>MGNYDSTPIAKSDRIKRLVDHLYAKMPEIEAARAELITESFKATEGQPVVMRKARAFEHILKNLPIIIRPEELIVGSTTIAPRGCQTYPEFSYEWLEAEFETVETRSADPFYISEETKKRLLAADAYWKGKTTSELATSYMAPETLRAMKHNFFTPGNYFYNGVGHVTVQYETVLAIGLNGVKEKVRKEMENCHFGDADYSTKMCFLESILISCDAVITYANRYAKMAEEMAEKETDAARRQELLTIARVCKNVPEFPAESFQEACQSFWFIQQVLQIESSGHSISPGRFDQYMYPYYEKDLKEGSLTREYAQELIDCIWVKLNDLNKCRDAASAEGFAGYSLFQNLIVGGQTVQGRDATNDLSFMCITASEHVFLPMPSLSIRVWHGSSKALLMRAAELTRTGIGLPAYYNDEVIIPALVHRGATMDEARNYNIIGCVEPQVPGKTDGWHDAAFFNMCRPLEMVFSNGYDNGEIASIQTGNVESFQSFDEFMEAYRKQMLYNIELMVNADNAIDYAHAKLAPLP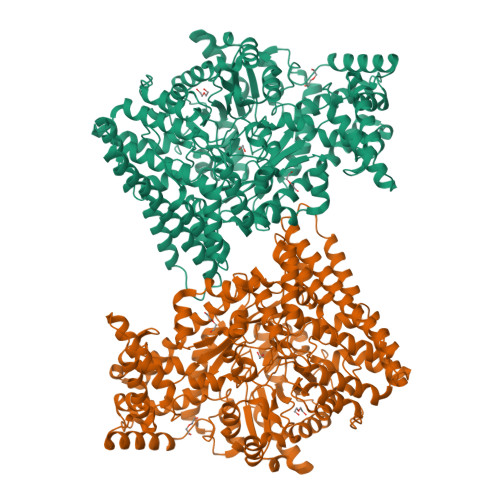FESCLVDDCIKRGMSAQEGGAIYNFTGPQGFGIANVADSLYTIKKLVFEEKRITMGELKKALEMNYGKGLDATTAGDIAMQVAKGLKDAGQEVGPDVIANTIRQVLEMELPEDVRKRYEEIHEMILELPKYGNDIDEVDELAREAAYFYTRPLETFKNPRGGMYQAGLYPVSANVPLGAQTGATPDGRLAHTPVADGVGPTSGFDISGPTASCNSVAKLDHAIASNGTLFNMKMHPTAMAGEKGLESFISLIRGYFDQQGMHMQFNVVDRATLLDAQAHPEKYSGLIVRVAGYSALFTTLSKSLQDDIIKRTEQADNR[2x]> MTGSNSHITILTLNINGLNSAIKRHRLASWIKSQDPSVCCIQETHLTCRDTHRLKIKGWRKIYQANGKQKKAGVAILVSDKTDFKPTKIKRDKEGHYIMVKGSIQQEELTILNIYAPNTGAPRFIKQVLSDLQRDLDSHTLIMGAFNTPLSTLDRSTRQKVNKDTQELNSALHQADLIDIYRTLHPKSTEYTFFSAPHHTYSKIDHIVGSKALLSKCKRTEIITNKLSDHSAIKLELR

The autonomous non-LTR retrotransposon long interspersed nuclear element-1 (LINE-1 or L1) is one the most abundant mobile elements in the human genome, comprising 17–20% of its content. ORF1p acts as a nucleic acid chaperone that binds L1 RNA, while ORF2p provides endonuclease (EN), reverse transcriptase (RT) and RNA-binding activities through three distinct functional domains. L1-EN initiates de novo L1 integration by producing a single-strand nick at a genomic site generally fitting the consensus target sequence 5′-TTTTT/AA-3′ (6,7,24,25). L1-EN belongs to the family of metal-dependent phosphohydrolases that includes apurinic/apyrimidinic endonuclease 1 (APE1) and DNase I, which are part of the exonuclease-endonuclease-phosphatase (EEP) domain superfamily.

Two mutations were introduced into L1-EN to facilitate crystallization of the enzyme complexed with DNA: D145A to prevent DNA cleavage and Y226K to alter crystal packing. The double mutant protein L1-EN-D145A/Y226K was readily crystallized in complex with two DNA substrates, dna14 and dna17, and structures were solved to a resolution of 2.8 Å. There is one DNA-protein complex in an asymmetric unit in crystals of L1-EN-D145A/Y226K with dna14 and two complexes in an asymmetric unit in crystals of the protein with dna17. Crystal packing is completely different in the case of the L1-EN/dna14 complex, where the terminal single nucleotide overhangs form Watson–Crick base pairs with symmetry-related dna14 molecules, thereby stabilizing the B-form helical conformation. In the complex of dna14 with L1-EN, we observed extended electron density around the A+1 phosphate at the scissile bond. Instead, we modeled two alternative conformations for this phosphate group with one corresponding to the typical conformation expected for a B-form helix (as observed in both complexes with dna17) and another where coordinated rotation of torsion bonds moves the phosphate closer to the active site residues, while largely preserving the positions of both 3′ and 5′ deoxyriboses. Importantly, this rotation brings the scissile bond phosphate group closer to active site amino acids Glu43 and Asp145. Thus, the observed rotation brings the scissile phosphate into a position favorable for nucleophilic attack and the proposed transition state (see details below). In the alternative conformation of dna14 bound to L1-EN, the rotated-out phosphate group is even closer to Glu43. Our structural analysis of the L1-EN-dna14 complex revealed rotation of the scissile bond phosphate group leading to two distinct states for the nucleophilic attack and a subsequent transition state.>MQTQVEDSAKPIVDPHDIDPKLVQKLANDALVWCSLRGLLVGDRNSERSGTVPGVDMVHAPVALIPMSFPESHWKQACEVAPIFNELVDRVSQDGEFLQQSLSRTRKVDPFTSRLLEIHSKMLEINKIEEIRLGLHRSDYMLDEQTKLLLQIELNTISSSFPGLSCLVSELHRSLLQQYREDIASDPNRIPANNAVNQFAEALAKAWNEYGDPRAVIMFAVQAEERNMYDQHWLSASLRERHQVTTIRKTLAEIDALGELQQDGTLVVDGQAVAVIYFRAGYAPSDYNSESEWKARLLMEQSRAVKCPSISYHLAGSKKIQQELAKPNVLERF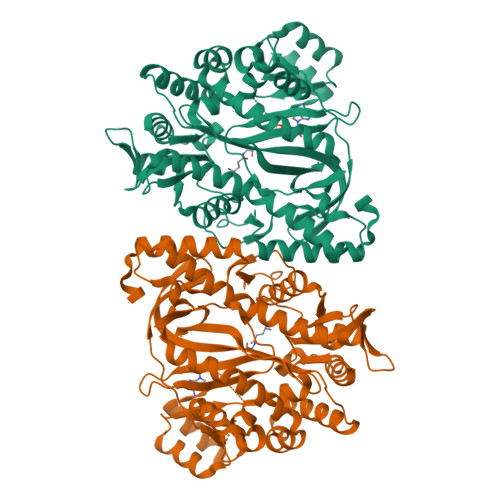LENKDDIAKLRKCFAGLWSLDESDIVKDAIDRPELYVMKPQREGGGNNIYGEDVRDALLKLQKEGTGSDAAYILMQRIFPKISHSILMREGISHKEQTISELGIYGTYLRNKTEVVINQQAGYLMRTKVSSSNEGGVAAGFAVLDSIYLV[6x]>MTDMRGTGQGLNLVDSVYERLLA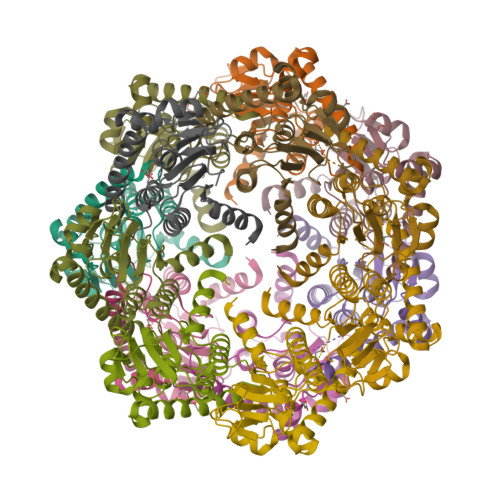ERIIFLGSQVDDDIANRLCAQILLLSAEDPTKDIHLYINSPGGSISAGMAIYDTMVLAPCDIATYAMGMAASMGEFLLAAGTKGKRYALPHARILMHQPLGGVTGSAADIAIQAEQFAVIKKEMFRLNAEFTGQPIERIEADSDRDRWFTAQEALEYGFVDHIITSASVNGEGPGAGLDKAAAHHHHHHHHHH[7x]> GPGSASCLELALEGERLCKSGDCRAGVSFFEAAVQVGTEDLKTLSAIYSQLGNAYFYLHDYAKALEYHHHDLTLARTIGDQLGEAKASGNLGNTLKVLGNFDEAIVCCQRHLDISRELNDKVGEARALYNLGNVYHAKGKSFGCPGPQDTGEFPEDVRNALQAAVDLYEENLSLVTALGDRAAQGR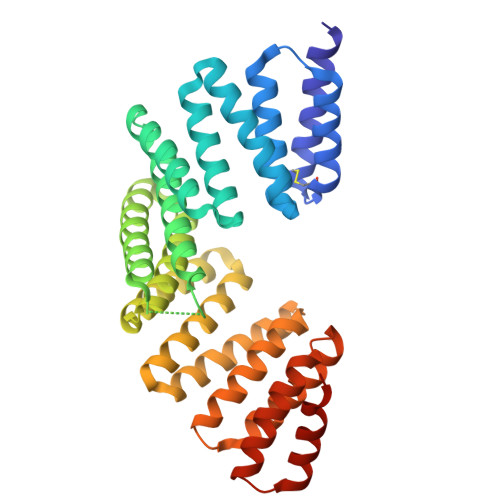AFGNLGNTHYLLGNFRDAVIAHEQRLLIAKEFGDKAAERRAYSNLGNAYIFLGEFETASEYYKKTLLLARQLKDRAVEAQSCYSLGNTYTLLQDYEKAIDYHLKHLAIAQELKDRIGEGRACWSLGNAYTALGNHDQAMHFAEKHLEISREVGD> MDLKILSLATDKTTDKLQEFLQTLKDDDLASLLQNQAVKGRAVGTLLRAVLKGSPCSEEDGALRRYKIYSCCIQLVESGDLQQDVASEIIGLLMLEVHHFPGPLLVDLASDFVGAVREDRLVNGKSLELLPIILTALATKKEVLACGKGDLNGEEYKRQLIDTLCSVRWPQRYMIQLTSVFKDVCLTPEEMNLVVAKVLTMFSKLNLQEIPPLVYQLLVLSSKGSRRSVLDGIIAFFRELDKQHREEQSSDELSELITAPADELYHVEGTVILHIVFAIKL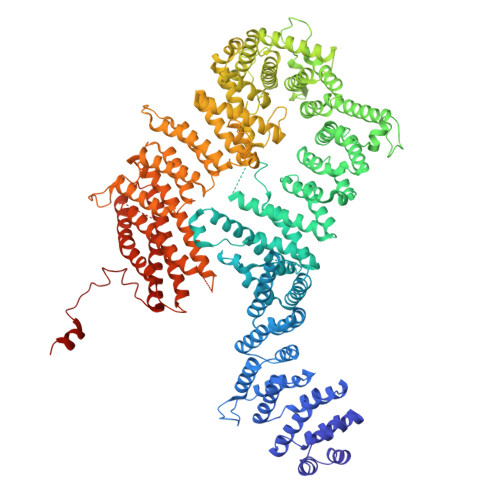DCELGRELLKHLKAGQQGDPSKCLCPFSIALLLSLTRIQRFEEQVFDLLKTSVVKSFKDLQLLQGSKFLQTLVPQRTCVSTMILEVVRNSVHSWDHVTQGLIEFGFILMDSYGPKKILDGKAVEIGTSLSKMTNQHACKLGANILLETFKIHEMIRQEILEQVLNRVVTRTSSPINHFLDLFSDIIMYAPLILQNCSKVTETFDYLTFLPLQTVQGLLKAVQPLLKISMSMRDSLILVLRKAMFASQLDARKSAVAGFLLLLKNFKVLGSLPSSQCTQSIGVTQVRVDVHSRYSAVANETFCLEIIDSLKRSLGQQADIRLMLYDGFYDVLRRNSQLASSIMQTLFSQLKQFYEPEPDLLPPLKLGACVLTQGSQIFLQEPLDHLLSCIQHCLAWYKSRVVPLQQGDEGEEEEEELYSELDDMLESITVRMIKSELEDFELDKSADFSQNTNVGIKNNICACLIMGVCEVLMEYNFSISNFSKSKFEEILSLFTCYKKFSDILSEKAGKGKAKMTSKVSDSLLSLKFVSDLLTALFRDSIQSHEESLSVLRSSGEFMHYAVNVTLQKIQQLIRTGHVSGPDGQNPDKIFQNLCDITRVLLWRYTSIPTSVEESGKKEKGKSISLLCLEGLQKTFSVVLQFYQPKVQQFLQALDVMGTEEEEAGVTVTQRASFQIRQFQRSLLNLLSSEEDDFNSKEALLLIAVLSTLSRLLEPTSPQFVQMLSWTSKICKEYSQEDASFCKSLMNLFFSLHVLYKSPVTLLRDLSQDIHGQLGDIDQDVEIEKTDHFAVVNLRTAAPTVCLLVLSQAEKVLEEVDWLIAKIKGSANQETLSDKVTPEDASSQAVPPTLLIEKAIVMQLGTLVTFFHELVQTALPSGSCVDTLLKGLSKIYSTLTAFVKYYLQVCQSSRGIPNTVEKLVKLSGSHLTPVCYSFISYVQNKSSDAPKCSEKEKAAVSTTMAKVLRETKPIPNLVFAIEQYEKFLIQLSKKSKVNLMQHMKLSTSRDFKIKGSVLDMVLREDEEHHHHHH> SSEKEYVEMLDRLYSKLPEKGRKEGT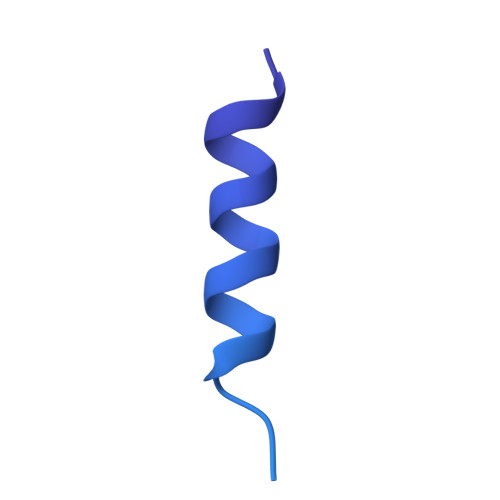QSLPNMIILNIGNTTIIRNFAEYCDRIRREDKICMKYLLKELAAPGNVDDKGELVIQGKFSSQVINTLMERFLKAYVECSTCKSLDTILKKEKKSWYIVCLACGAQTPVKPL4-[2,6-bis(fluoranyl)-4-(3-morpholin-4-ylpropylcarbamoylamino)phenoxy]-~{N}-[(4-methyl-1,2,5-oxadiazol-3-yl)methyl]-1~{H}-pyrrolo[2,3-b]pyridine-3-carboxamide 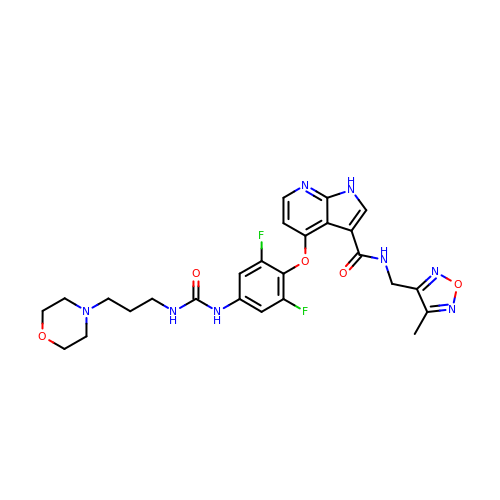| C26 H28 F2 N8 O5 | SENYRIRBXVWYED-UHFFFAOYSA-N>[4x]AMTDIPDRKEAVISLWPEFAKAIVSGKKTVEFRRRIPLPALSARIWIF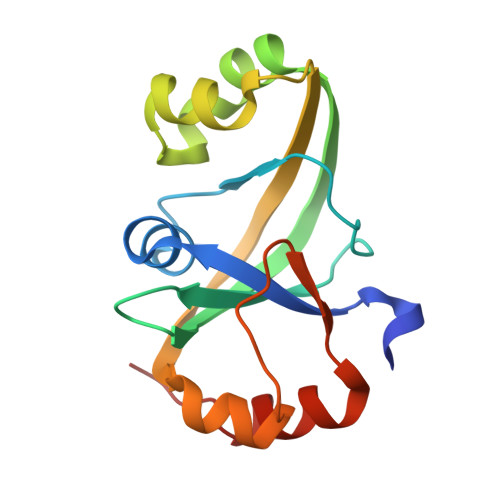ATRPVKSVIGFAYLEAIVQGDVNTLWSRYGREAFLSEQQYRDYFEGTEKATAFLLRDHQPIRPINLDQLKEIRANFQPPQSLTWLRKEETQKLVSLTSQVE>GAMTAEALELGRQQAQLLRRSVRRFSTDPVPGDLVEAAVAEALTAPAPHHTRPTRFVWLQTPAIRARLLDRMKDKWRSDLTSDGLPADAIERRVARGQILYDAPEVVIPMLVPDGAHSYPDAARTDAEHTMFTVAVGAAVQALLVALAVR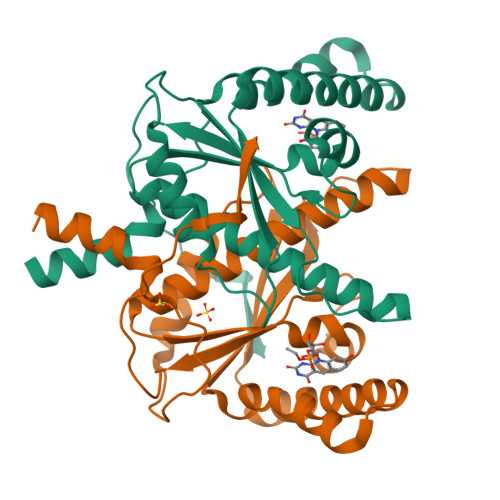GLGSCWIGSTIFAADLVRDELDLPVDWEPLGAIAIGYADEPSGLRDPVPAADLLILK[4x]>[2x]GNADELYK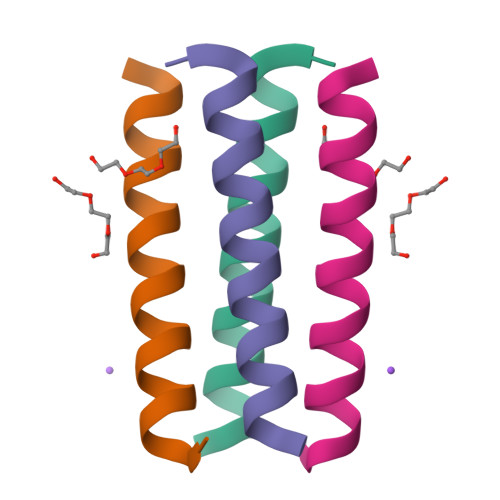EXEDLQERXRKLRKKXRSG> MKLTDGQIRINHVS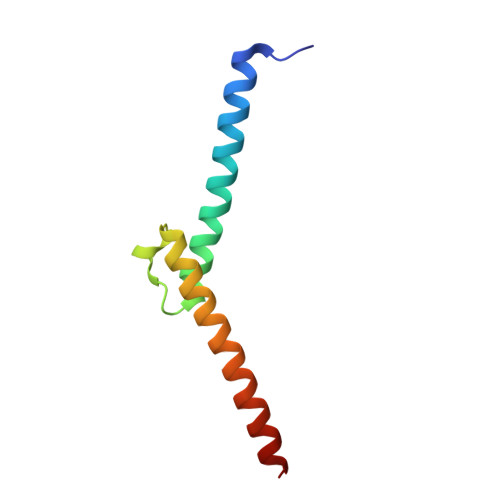SEKKRRELERAIFDELVAVVPDLQPQESRSELIIYLKSLSYLSWLYERNEKLRKQIIAKHE> MAEGEITTFTALTEKFNLPPGNYKKPKLLYCSNGGHFLRILPDGTVDGTRDRSDQHI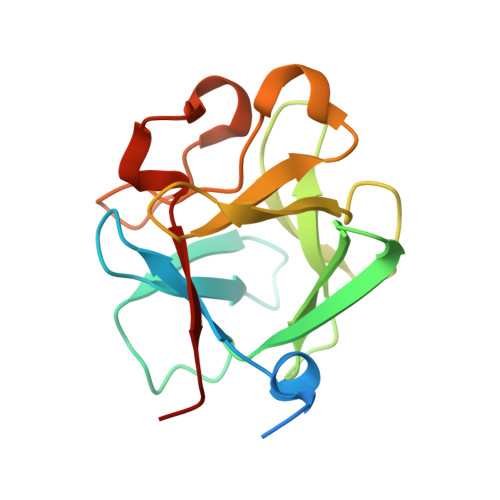QLQLSAESVGEVYIKSTETGQYLAMDTDGLLYGSQTPNEECLFLERLEENHYNTYISKKHAEKNWFVGLKKNGSCKRGPRTHYGQKAILFLPLPVSSD> LVEA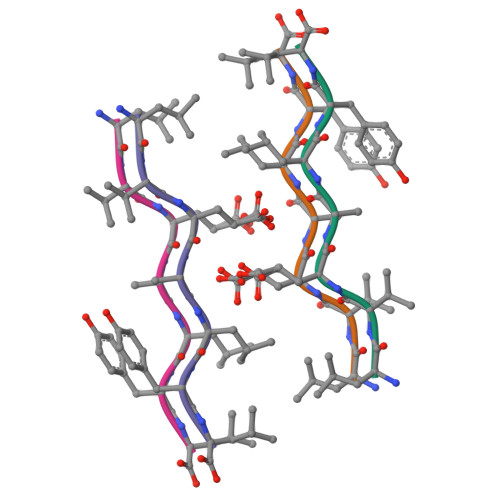LYL>MLTQKTKDIVKATAPVLAEHGYDIIKCFYQRMFEAHPELKNVFNMAHQEQGQQQQALARAVYAYAENIEDPNSLMAVLKNIANKHASLGVKPEQYPIVGEHLLAAIKEVLGNAATDDIISAWAQAYGNLADVLMGMESELYERSAEQPGGWKGWRTFVIREKRPESDVITSFILEPADGGPVVNFEPGQYTSVAIDVPALGLQQIRQYSLSDMPNGRTYRISVKREGGGPQPPGYVSNLLHDHVNVGDQVKLAAPYGSFHIDVDAKTPIVLISGGVGLTPMVSMLKVALQAPPRQVVFVHGARNSAVHAMRDRLREAAKTYENLDLFVFYD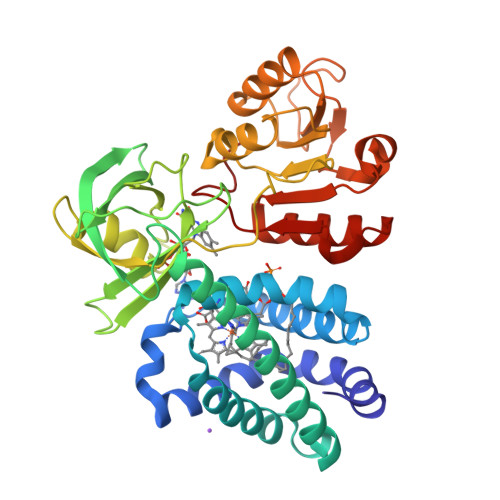QPLPEDVQGRDYDYPGLVDVKQIEKSILLPDADYYICGPIPFMRMQHDALKNLGIHEARIHYEVFGPDLFAE[2x]>[4x]MNSNKELMQRRSQAIPRGVGQIHPIFADRAENCRVWDVEGREYLDFAGGIAVLNTGHLHPKVVAAVEAQLKKLSHTCFQVLAYEPYLELCEIMNQKVPGDFAKKTLLVTTGSEAVENAVKIARAATKRSGT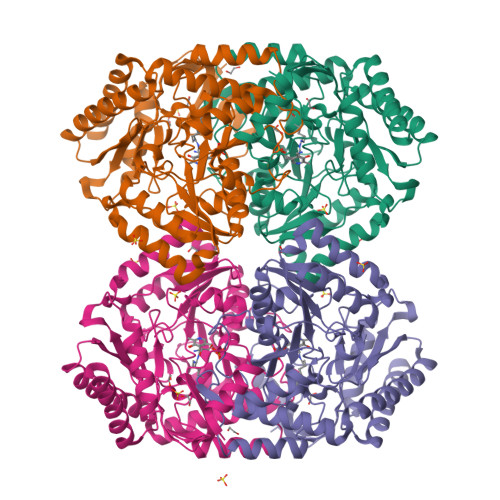IAFSGAYHGRTHYTLALTGKVNPYSAGMGLMPGHVYRALYPCPLHGISEDDAIASIHRIFKNDAAPEDIAAIVIEPVQGEGGFYASSPAFMQRLRALCDEHGIMLIADEAQSGAGRTGTLFAMEQMGVAPDLTTFAKSIAGGFPLAGVTGRAEVMDAVAPGGLGGTYAGNPIACVAALEVLKVFEQENLLQKANDLGQKLKDGLLAIAEKHPEIGDVRGLGAMIAIELFEDGDHNKPDAKLTAEIVARARDKGLILLSCGPYYNVLRILVPLTIEDAQIRQGLEIISQCFDEAKQ>HDKVVVLEAKNGNVTFDHKKHAGVKGECKACHETEAGGKIAGMGKDWAHKTCTGCHKEMGKGP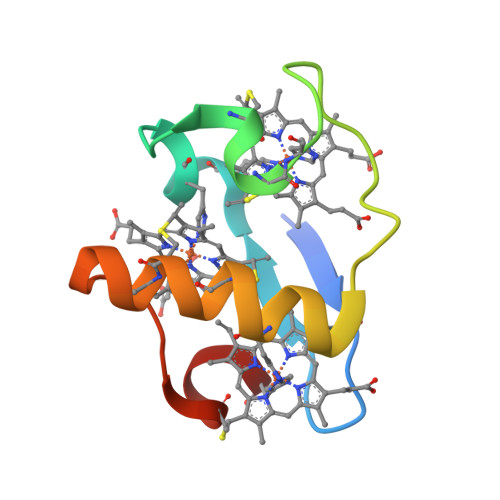TKCGECHKK[2x]N-[(1S,2S)-1-(3,5-difluorobenzyl)-2-hydroxy-2-{(2R)-4-[(3-methylphenyl)sulfonyl]piperazin-2-yl}ethyl]-3-{[(2R)-2-(methoxymethyl)pyrrolidin-1-yl]carbonyl}-5-methylbenzamide 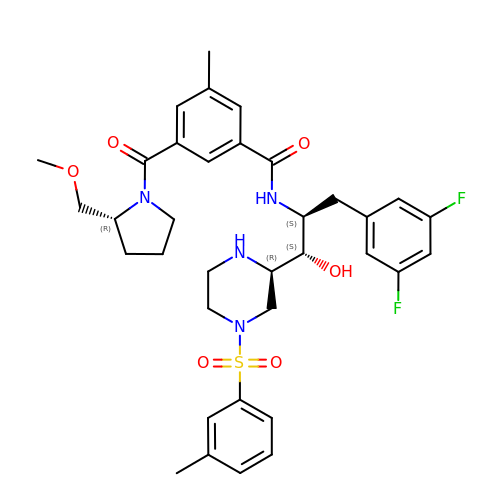| C35 H42 F2 N4 O6 S | CQQMWBPWYUPVOC-PPESYSCFSA-N However, this belief has recently been challenged by the discovery of a dsRBD serving as a major tRNA binding module for human dihydrouridine synthase 2 (hDus2), a flavoenzyme that catalyzes synthesis of dihydrouridine within the complex elbow structure of tRNA. Dus2 is found in all eukaryotes and catalyzes formation of dihydrouridine 20 in tRNA. However, in stark contrast, we showed that, despite the presence of a HD domain, hDus2 and by inference from the sequences probably all animal ones instead use a novel extended dsRBD version flanked by a peculiar N-terminal extension (NTE) and C-terminal extension (CTE) to provide the major binding sites for tRNA substrate. By solving the crystal structure of this dsRBD in complex with a dsRNA together with extensive characterizations of its interaction with tRNA using mutagenesis, NMR and SAXS, we establish that while hDus2 dsRBD retains a conventional dsRNA recognition capability, the presence of an N-terminal extension appended to the canonical domain provides additional residues for binding tRNA in a structure-specific mode of action.

Mutation of the conserved residue, K371, reduced the binding by ∼8-fold while that of K419 or K420 by >4-fold respectively, demonstrating the importance of interactions engaging both α1 and α2 helices. In order to substantiate the idea of a synergistic effect due to NTE, we tested the effect of a double mutation in the canonical dsRBD. We chose to produce K419A–K420A because of the important role played by these residues (see above). The double mutant led to a ∼17-fold decrease in the apparent affinity for tRNA, rather hitting for an additive mode of action of these residues. Similarly to R361A–R362A, this effect is purely attributed to loss of positive charges since the structure of K419A–K420A is similar to that of the wild type (RMSD of 0.6 Å over 82 Cα).

> MTSEQTGEPAEDTSGVIKMAVKFDRRAYPAQITPKMCLLEWCRREKLAQPVYETVQRPLDRLFSSIVTVAEQKYQSTLWDKSAALAEQAAAIVCLRSQGLPEGRLGEESPSLHKHHHHHH> KKKV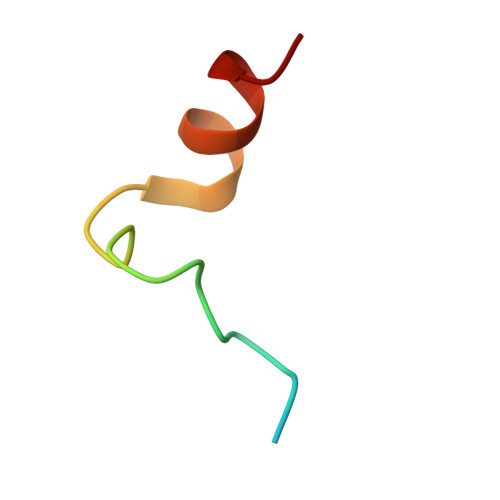RKYWDVPPPGFEHITPMQYKAMQA> GAMDPRKGYKVLAIETSCDDTCVSVLDRFSKSAAPNVLANLKDTLDSIDEGGIIPTKAHIHHQARIGPLTERALIESNAREGIDLICVTRGPGMPGSLSGGLDFAKGLAVAWNKPLIGVHHMLGHLLIPRMGTNGKVPQFPFVSLLVSGGHTTFVLSRAIDDHEILCDTIDIAVGDSLDKCGRELGFKGTMIAREMEKFINQDINDQDFALKLEMPSPLKNSASKRNMLSFSFSAFITALRTNLTKLGKTEIQELPEREIRSIAYQVQESVFDHIINKLKHVLKSQPEKFKNVREFVCSGGVSSNQRLRTKLETELGTLNSTSFFNFYYPPMDLCSDNSIMIGWAGIEIWESLRLVSDLDICPIRQWPLNDLLSVDGWRTDQL

N6-threonylcarbamoyladenosine (t6A) is one of the 15 universally conserved tRNA modifications found in all three domains of life. With the sole exception of bacterial initiator tRNAfMet, t6A is present at position 37 of the anti-codon stem loop of all tRNAs with ANN recognizing anticodons (N being any nucleotide). This modification serves to strengthen the codon–anticodon interaction and promote translational fidelity by the ribosome. Toward this end, we show that yeast Sua5 and Qri7 (the mitochondrial paralogue of Kae1) are sufficient for t6A biosynthesis in vitro. In summary, the eukaryotic t6A biosynthesis system functions first through Sua5, which generates TCA using its adenylation function and then secondly through Qri7, which binds to TCA to conjugate the threonyl-carbamoyl moiety onto directly bound tRNA substrates.

To shed light onto the structural basis for the unique functional properties of Qri7, we solved the structure of yeast Qri7. Qri7 exhibits the prototypical bilobal structure with its catalytic region sandwiched between subdomains I and II. Crystal structures of Kae1 orthologues (like ASKHA fold proteins in general) display variability in interlobe closure, and the Qri7 structure is notable in adopting the most open configuration reported to date for a Kae1 orthologue. Projection of conservation onto the Qri7 structure identified a large contiguous surface emanating from the catalytic cleft. A portion of the conserved surface was accounted for by the expected binding sites of TCA and phosphate coordinating metal ions. The binding of acceptor substrate (tobramycin) in the evolutionarily related TobZ crystal structure identifies these unaccounted for conserved surfaces at the tips of subdomains I and II as the possible tRNA substrate-binding surface. Application of crystallographic symmetry to the Qri7 monomer structure revealed a dimer configuration with a large (2087.5 Å2) hydrophobic buried surface, which is partially conserved across Qri7 orthologues. Remarkably, the Qri7 dimerization surface is the same surface used by archaeal and eukaryotic Kae1 proteins to bind Pcc1, a dimerization module within KEOPS and the same surface used by the bacterial orthologue YgjD to bind YeaZ. We confirmed that Qri7 forms homodimers in solution with a dissociation constant of 60 nM by equilibrium analytical ultracentrifugation. The R104A and K130A mutants displayed a dimerization dissociation constant of 3.0 ± 0.3 μM and 2.5 ± 0.2 μM, respectively. These results confirm that Qri7 forms homodimers in solution through the same binding mode revealed in the crystal structure.> MAMSNMTYNNVFDHAYEMLKENIRYDDIRDTDDLHDAIHMAADNAVPHYYADIFSVMASEGIDLEFEDSGLMPDTKDVIRILQARIYEQLTIDLWEDAEDLLNEYLEEVEEYEEDE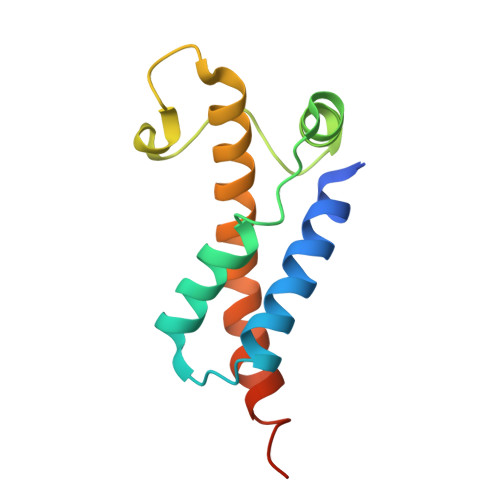E> TASPSALADE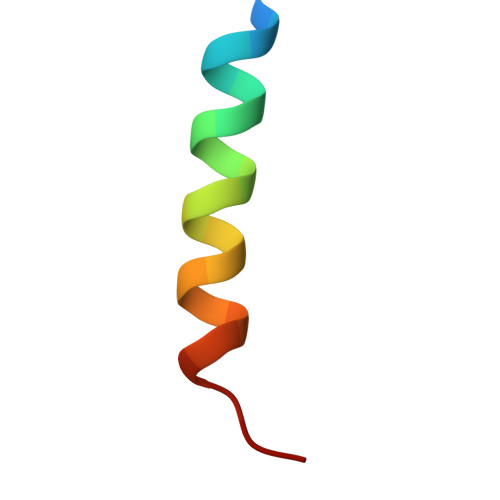LEQLAYEVEHLSS> GSHMSAPGPLVFTALSPDSLQLSWERPRRPNGDIVGYLVTCEMAQGGGPATAFRVDGDSPESRLTVPGLSENVPYKFKVQARTTEGFGPEREGIITIES

Integrin α6β4 is a major component of hemidesmosomes that mediate the stable anchorage of epithelial cells to the underlying basement membrane. The β4 subunit only pairs with the α6 subunit to form the α6β4 integrin, which is a laminin receptor required for maintaining the integrity of epithelia. The third and fourth fibronectin type III domains (FnIII-3,4) of integrin β4 mediate binding to the hemidesmosomal proteins BPAG1e and BPAG2, and participate in signalling. The crystal structures of the individual FnIII-3 and FnIII-4 domains were solved and the relative arrangement of the FnIII domains was elucidated by combining DEER with site-directed spin labelling.

The structure of the FnIII-4 domain (1572–1666) was refined against data extending to 1.50 Å resolution; the FnIII-4 crystals contain a single protein molecule in the asymmetric unit. In contrast to FnIII-3, the region around Y1642 is mostly uncharged. In contrast to Y1494 and Y1526 in FnIII-3, Y1642 in FnIII-4 sits in a wider pocket surrounded by uncharged residues. Therefore, phosphorylation of Y1642 is less likely to destabilize FnIII-4 and correlates with a minor role of Y1642 in the recruitment of Shc.> SSHKFTVVVLRATKVTKGAFGDMLDTPDPYVELFISTTPDSRKRTRHFNNDINPVWNETFEFILDPNQENVLEITLMDANYVMDETLGTATFTVSSMKVGEKKEVPFIFNQ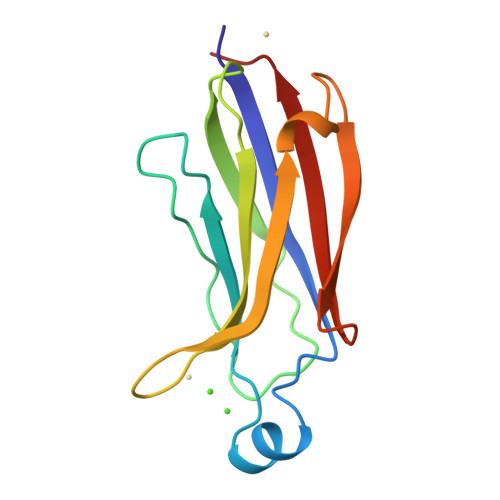VTEMVLEMSLEVASS>GLEVDNNSLLRNIYSTIVYEYSDIVIDFKTSHNLVTKKLDVRDARDFFINSEMDEYAANDFKTGDKIAVFSVPFDWNYLSKGKVTAYTYGGITPYQKTSIPKNIPVNLWINGKQISVPYNEISTNKTTVTAQEIDLKVRKFLIAQHQLYSSG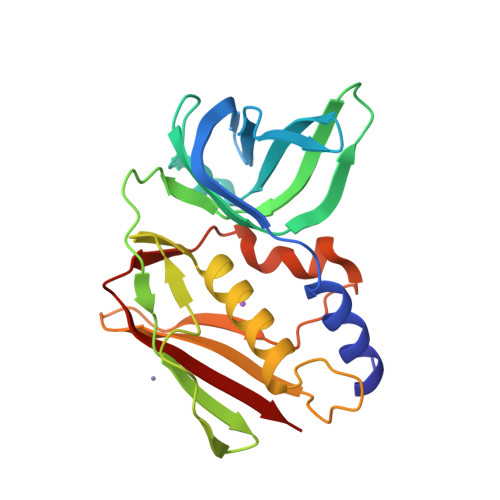SSYKSGRLVFHTNDNSDKYSFDLFYVGYRDKESIFKVYKDNKSFNIDKIGHLDIEIDS[2x]> MRPEPGGCCCRRTVRANGCVANGEVRNGYVRSSAAAAAAAAAGQIHHVTQNGGLYKRPFNEAFEETPMLVAVLTYVGYGVLTLFGYLRDFLRYWRIEKCHHATEREEQKDFVSLYQDFENFYTRNLYMRIRDNWNRPICSVPGARVDIMERQSHDYNWSFKYTGNIIKGVINMGSYNYLGFARNTGSCQEAAAKVLEEYGAGVCSTRQEIGNLDKHEELEELVARFLGVEAAMAYGMGFATNSMNIPALVGKGCLILSDELNHASLVLGARLSGATIRIFKHNNMQSLEKLLKDAIVYGQPRTRRPWKKILILVEGIYSMEGSIVRLPEVIALKKKYKAYLYLDEAHSIGALGPTGRGVVEYFGLDPEDVDVMMGTFTKSFGASGGYIGGKKELIDYLRTHSHSAVYATSLSPPVVEQIITSMKCIMGQDGTSLGKECVQQLAENTRYFRRRLKEMGFIIYGNEDSPVVPLMLYMPAKIGAFGREMLKRNIGVVVVGFPATPIIESRARFCLSAAHTK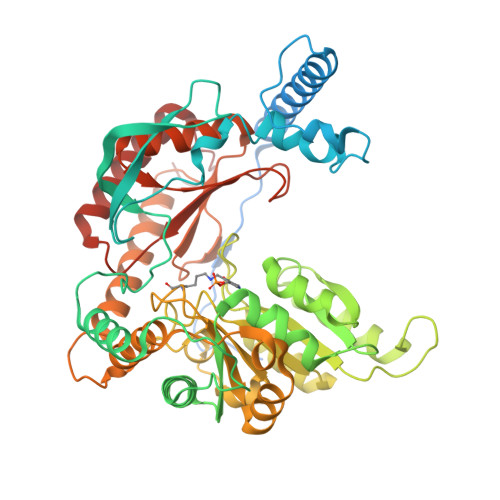EILDTALKEIDEVGDLLQLKYSRHRL>DYKDDDDKLHSQANLMRLKSDLFNRSPMYPGPTKDDPLTVTLGFTLQDIVKADSSTNEVDLVYYEQQRWKLNSLMWDPNEYGNITDFRTSAADIWTPDITAYSSTRPVQVLSPQIAVVTHDGSVMFIPAQRLSFMCDPTGVDSEEGATCAVKFGSWVYSGFEIDLKTDTDQVDLSSYYASSKYEILSATQTRQVQHYSCCPEPYIDVNLVVKFRERRA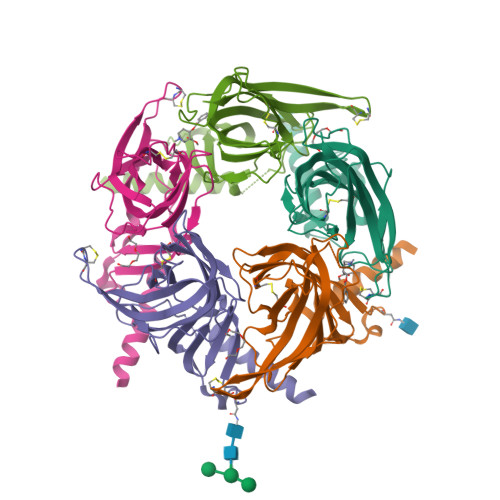GNGFFRNLFDSR[5x]>[3x]MEMLTKFESRSSRAKGVAFHPTQPWILTSLHNGRIQLWDYR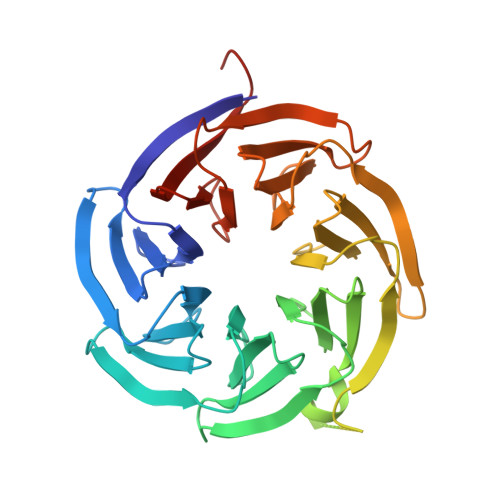MGTLLDRFDGHDGPVRGIAFHPTQPLFVSGGDDYKVNVWNYKSRKLLFSLCGHMDYVRVCTFHHEYPWILSCSDDQTIRIWNWQSRNCIAILTGHSHYVMCAAFHPSEDLIVSASLDQTVRVWDISGLRMKNAAPVSMSKEDQKAQAHNSKSNDKKGSTDAIVKFVLEGHDRGVNWCAFHPTLPLILSAGDDRLVKLWRMTASKAWEVDTCRGHFNNVSCCLFHPHQELILSASEDKTIRVWDLNRRTAVQTFRRDNDAFWFITVHPKLNLFAAAHDSGVMVFKLESAWSHPQFEK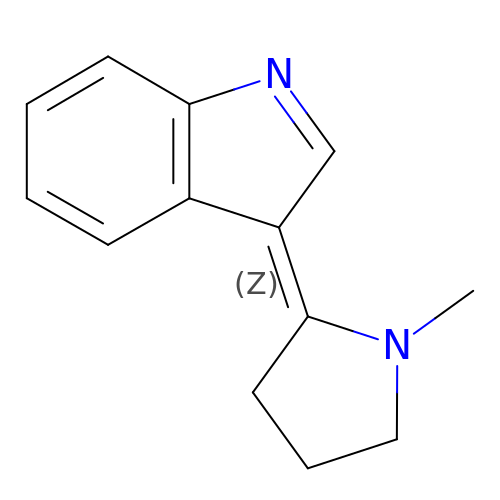(3~{Z})-3-(1-methylpyrrolidin-2-ylidene)indole | C13 H14 N2 | HNNADWWHLOZSTI-ACCUITESSA-N>[4x]SMGKAPVDPECTAKVGKAHVYCEGNDVYDVMLNQTNLQFNNNKYYLIQLLEDDAQRNFSVWMRWGRVGKMGQHSLVACSGN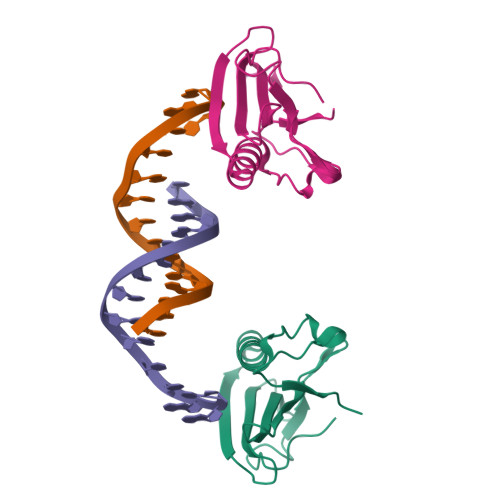LNKAKEIFQKKFLDKTKNNWEDREKFEKVPGKYDMLQMDYATNTQDEEET>[2x]GAMGSTTPIADIQQGISKYLDALNVFCRASTFLTDLFSTVFRNSHYSKAATQLKDVQEHVMEAASRLTSAIKPEIAKMLMELSAGAANFTDQKEFSLQDIEVLGRCF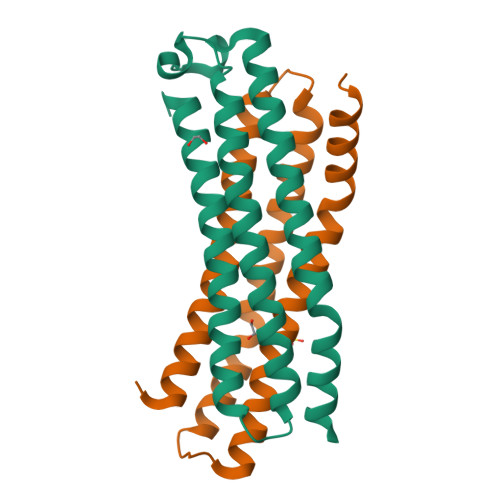LTVVQVHFQFLTHALQKVQPVAHSCFAEVIVPEKKNS>[6x]MRTLLIRYILWRNDNDQTYYNDDFKKLMLLDELVDDGDVSTLIKNMRMTLSDGPLLDRLNYPVNNIEDAKRMIAISAKVARDIGERSEIRWEESFTILFRMIETYFDDLMIDLYGEKLEHHHHHH

VACV protein N1 is an intracellular virulence factor that is expressed early during infection and modulates innate immunity by at least two strategies: preventing apoptosis and inhibiting NF-κB activation. N1 is a Bcl-2-like protein that contains a surface groove similar to those in cellular anti-apoptotic Bcl-2 proteins that bind the BH3 motif of pro-apoptotic Bcl-2 members. The VACV Bcl-2-like proteins N1, B14 and A52 all form dimers via a common surface comprising alpha helices 1 and 6 (the ‘1–6 face’). Biochemical and structural analysis of these mutants demonstrates that the anti-apoptotic activity of N1 relies on a hydrophobic groove on the surface of the protein and that the anti-NF-κB activity requires an intact dimer interface.

By analogy with VACV proteins A52 and B14, which have the surface groove filled by bulky amino acid residues and do not inhibit apoptosis, we introduced the bulky residue tyrosine at positions R58, Q61 and R71 in an attempt to ‘fill’ the N1 groove and thereby exclude BH3-peptide binding. To determine if the point mutations introduced in N1 generated unanticipated structural changes, R58Y, Q61Y and R71Y N1 were expressed in bacteria, purified to homogeneity and their structures determined at 3.0–3.1 Å resolution. All three mutants crystallized in the same space group as wild-type N1 and the overall structures of all three closely resembled the wild-type protein (0.21–0.39 Å r.m.s. deviation over 108 Cα atoms). For both the R58Y and Q61Y mutants, the tyrosine residue protruded into the groove in a manner likely to reduce BH3 peptide binding. While WT N1 and the groove-filling mutants (R58Y, Q61Y, R71Y) were all dimeric, the I6E mutant was almost exclusively monomeric. Introduction of the groove-filling mutations R58Y and Q61Y abolished the ability of N1 to prevent apoptosis, while mutants R71Y and I6E inhibited STS-induced apoptosis as strongly as WT N1. In this assay, both WT and I6E mutant N1, where the groove is intact, interacted with HA-tagged Bad, whereas groove-filling Q61Y mutant N1, as well as A52, failed to immunoprecipitate with Bad. Likewise, when untagged Bid was co-expressed in cells, Q61Y mutant was unable to interact with Bid, whereas R71Y mutant, as well as WT N1, still immunoprecipitated Bid. In contrast, mutant Q61Y which has an occluded surface groove no longer binds Bid or Bad and no longer inhibits apoptosis. Expression of WT N1 decreased NF-κB activation significantly, as did expression of the groove mutants.> DYKDDDDLEVLFQGPGGSSAPARPNWLAYDWGLVFLVAAIVALGFVNLGSAAPDPVLLYRQSVALGLGLLLAFLLQFLSRRRLFGLAYPLYGASLLLLALVLVVGREINGARAWFVLGPLQFQPLELAKLGLLLALAKALEGRPIARVW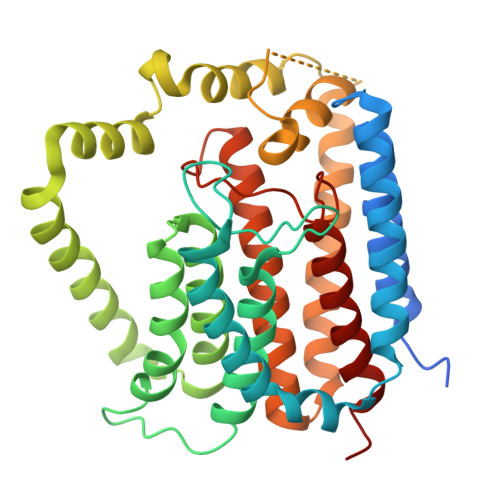DYALPALLTLPVVGLLLLQPDLGGALVVLFGVFVVVFVRGLPWRHLLVGLFALALLVPTAVWPNLKPYQRERVLIVLDPYRDPLGQGFQVIQSTIAIGSGGLFGKGYGQGTQAQLGFIPFRHTAFVFSVWAEEWGFVGVVGLLGLYGLLLARLFALALACPRLSDRLFLSGFAGMLGFQVVVNLGVALGVMPVTGLTLPLFSYGGSSLIATLAGLGLVLLVHRDRYQD2-[diethyl(methyl)-$l^{4}-azanyl]ethyl 4-[(2-octoxyphenyl)carbonylamino]benzoate | C29 H43 N2 O4 | 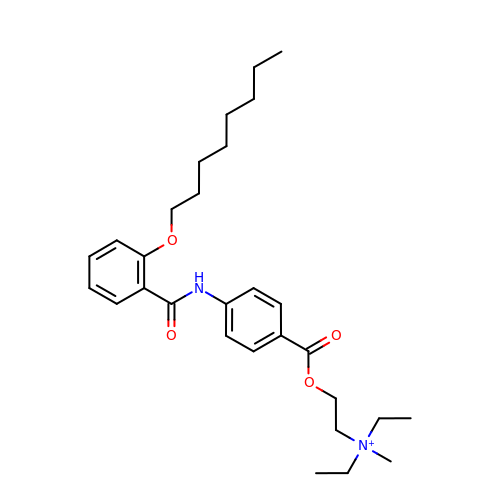NQHNLNLJPDMBFN-UHFFFAOYSA-O> LYTGAVPRANRIVQQLVEAGADLANIRTMFRNMLRGEEMILSRAEQNVFLQHFPDMLPCGIDRNSEL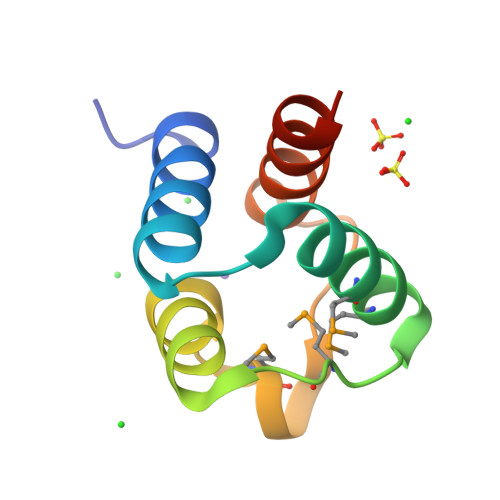AIALREALRRADSQQA> SNAYTVFIDPGHGGNDKGTESKTSNRYEKDLNLQIAKKLANKLSKQKDIQVVVSRTDDTYISLKDRAILANNSSADVLVSIHLNAEKNGNTATGIETWYRNKATDGSKELAQTVQSTIVSYVKVRDRGIVENNFEVLRESNMPAILI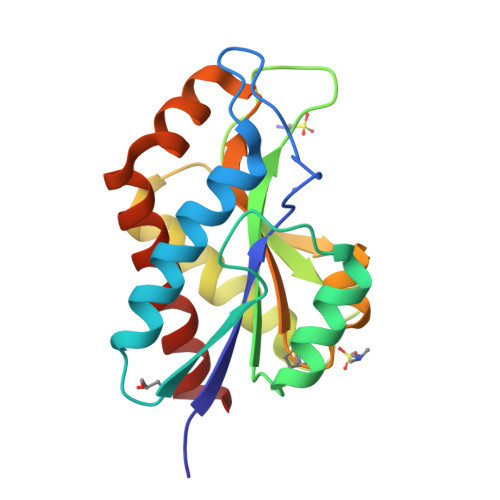ECGFLTTPSEEQKIINEKYQDQLAEGIVQGVLSYLDSKGNK>[6x]GSGAIGGNIVSHDDALLNTLAILQKELKSKEQEIRRLKEVIALKNKNTERLNDELI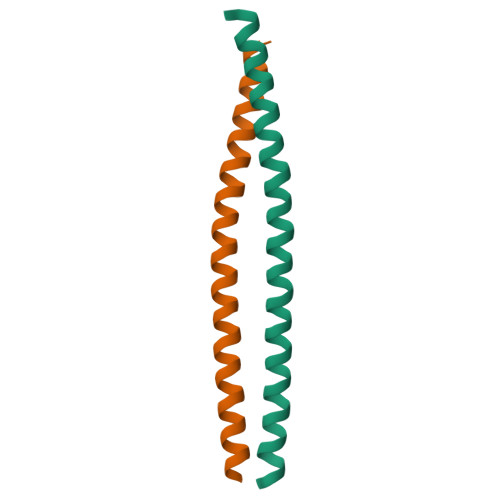SGTIENNVLQQKLSDLKKE4-[3-(2-azanylpyrimidin-4-yl)-1~{H}-indol-5-yl]-2-methyl-but-3-yn-2-ol 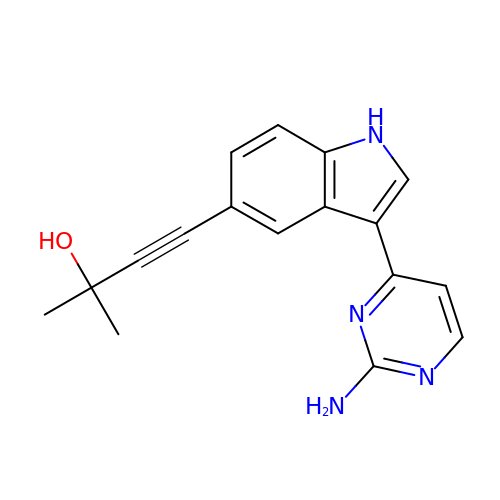| C17 H16 N4 O | YYAZUVAPGBAUDQ-UHFFFAOYSA-N[(2~{R})-1-(dimethylamino)-1-oxidanylidene-4-phenyl-butan-2-yl]azanium | C12 H19 N2 O | 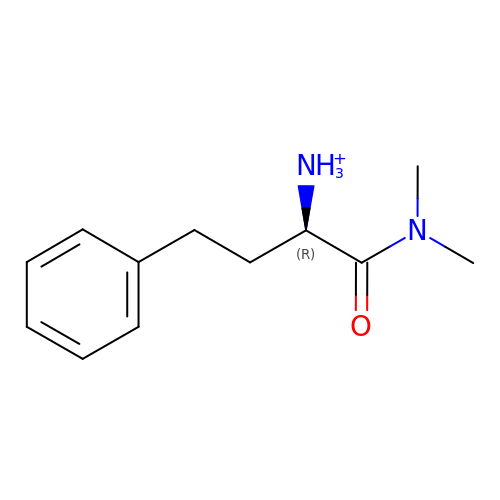QEESVUFHIWOBTA-LLVKDONJSA-O> MDTQTHLNFTQIKTVDELNQALVEAKGKPVMLDLYADWCVACKEFEKYTFSDPQVQKALADTVLLAANVTANDAQDVALLKHLNVLGLPTILFFDGQGQEHPQARVTGFMDAETFSAHLRDRQPGLVPRGSG

The transmembrane thiol:disulfide oxidoreductase DsbD is a three-domain protein responsible for shuttling electrons from the cytoplasm to the oxidizing periplasm of Gram-negative bacteria. Its central domain (tmDsbD) is located in the inner bacterial membrane and is flanked by two periplasmic globular domains (nDsbD, the N-terminal domain, and cDsbD, the C-terminal domain). cDsbD, like many proteins involved in periplasmic oxidative protein folding, adopts the more conventional Trx fold. Its role is very specific, to acquire reductant from tmDsbD and transfer it to nDsbD.

In this work we have found that replacing Gln-488 with an alanine residue, which cannot form a hydrogen bond or a salt bridge in the active site, has a dramatic effect on the pKa value of Cys-461. Despite the presence of reducing agent (TCEP) in the mother liquor, both proteins were found to be oxidized with a Cys-461–Cys-464 disulfide bond clearly present. The cysteine pair (Cys-461 and Cys-464), Asp-455, and Glu-468 of wild-type cDsbD overlay well with the same residues of Q488A-cDsbD. The only difference is that the side chain of Gln-488 is absent in Q488A-cDsbD and replaced by the much shorter alanine side chain. The carboxyl side chains of Asp-455 and Glu-468 in both wild-type and Q488A-cDsbD are oriented toward Cys-461 and remain in close proximity (<∼8 Å) to the N-terminal cysteine of the -CXXC- motif. The side chain solvent accessibilities of Asp-455 (9%) and Glu-468 (57%) in Q488A-cDsbD are comparable with those in wild-type cDsbD (7% for Asp-455 and 42% for Glu-468). In wild-type cDsbD, the hydrogen bond interaction with Gln-488 stabilizes the carboxylate group of Asp-455 and results in a pKa value of 5.8 or 6.7, depending on the oxidation state of the protein. In Q488A-cDsbD, the absence of this stabilizing interaction leads to a further elevation of the pKa value of Asp-455 to a point where it becomes indistinguishable from the pKa value of Cys-461. The phenomenon of microscopic pKa values occurs between Asp-455 and Cys-461 in Q488A-cDsbDred and, as a result, in a fraction of the protein molecule population Cys-461 has a pKa value of 7.6, which makes it significantly more reactive and prone to reoxidation compared with the wild-type domain. This was apparent when we measured the activity of this variant in the full-length protein in vivo; Q488A-DsbD was only ∼75% functional compared with wild-type-DsbD, consistent with part of the protein population being compromised.>[3x]AEIDEGVFETTATIDNGSFGTRTIRFETGRLALQAAGAVVAYLDDDNMLLSATTASKNPKEHFDFFPLTVDVEERMYAAGRIPGSFFRREGRPSTDAILTCRLIDRPLRPSFVDGLRNEIQIVVTILSLDPGDLYDVLAINAASASTQLGGLPFSGPIGGVRVALIDGTWVGFPTVDQIERAVFDMVVAGRIVEGDVAIMMVEAEATEN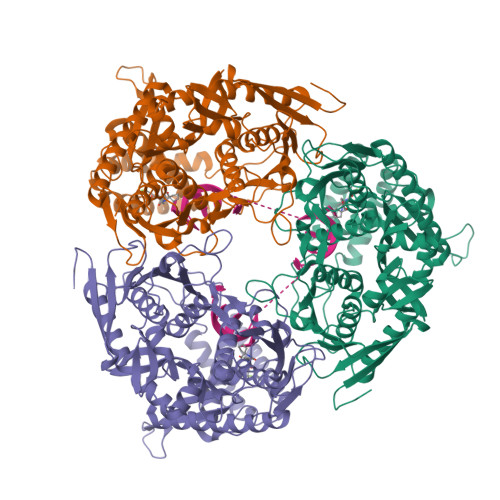VVELVEGGAQAPTESVVAAGLEAAKPFIAALCTAQQELADAAGKSGKPTVDFPVFPDYGEDVYYSVSSVATDELAAALTIGGKAERDQRIDEIKTQVVQRLADTYEGREKEVGAAFRALTKKLVRQRILTDHFRIDGRGITDIRALSAEVAVVPRAHGSALFERGETQILGVTTLDMIKMAQQIDSLGPETSKRYMHHYNFPPFSTGETGRVGSPKRREIGHGALAERALVPVLPSVEEFPYAIRQVSEALGSNGSTSMGSVCASTLALLNAGVPLKAPVAGIAMGLVSDDIQVEGAVDGVVERRFVTLTDILGAEDAFGDMDFKVAGTKDFVTALQLDTKLDGIPSQVLAGALEQAKDARLTILEVMAEAIDRPDEMSPYAPR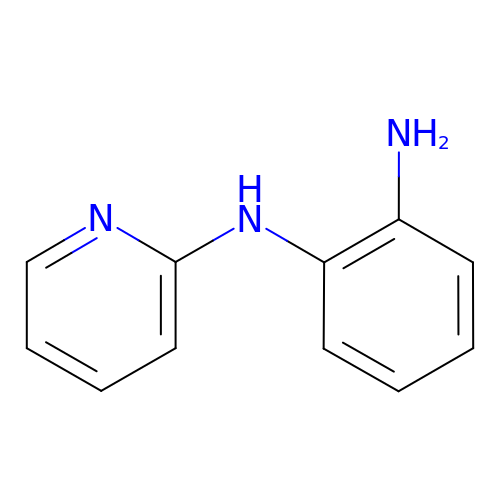~{N}2-pyridin-2-ylbenzene-1,2-diamine | C11 H11 N3 | SMNUYINHUNGHMQ-UHFFFAOYSA-N> MSKTLMLVKSGLAAGAMGGVALVAGTAQNVAPPPAALAPSYLVKTADSSCADPAWNAAAVYTGGQRVSYQNQTWQAKWWTQGNTPAAGDASPWQLIGQCGGGTPSDPPLVQVPPPTGNALCRPEALAQTQGVDVPYCAVYKQGGAEQLANGSRRRIIGYFTSWRTGKDGSPAYLASDIPWSKLTHINYAFAHVDGSNKLSVNETAPGNPATDMSWPGVAGAEMD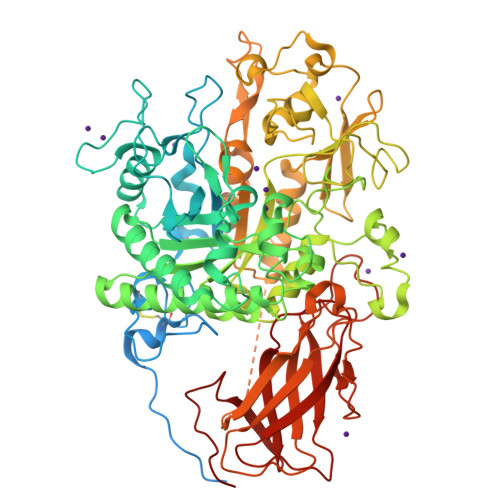ASLPYKGHFNLLTQYKRKYPGVKTLISVGGWAETGGYFDANGKRVASGGFYSMTVNADGTVNQAGINAFSDSAVAFLRKYGFDGVDIDFEYPTSMNNAGNPLDWTFSNARLGSLNKGYVALLQTLRDRLDRAAAQDGRYYQITAAVPASGYLLRGMETFQGLKYLDFVNVMSYDLHGAWNRFVGPNAALYDDGKDAELAFWNVYSTPQYGNIGYLNTDWAYHYYRGGLPASRVNMGVPYYTRGWKNVSGGSNGLWGSSVGSNCPAGLTECGDGAVGIDNIWHDLDDSGKEIPGGSNPMWHAKNLEKGLAGSYLAAYGIDPTLPINQLTGSYQRNYNGALAAPWLWNAGKKVFLSTEDEQSIAQKAAWIDANNVGGVMFWELAGDYDWKAQRNNGQGEYFIGTTLTSLLYNTFSQPPKVSARRADAAPAPTAAIDVGFSLGGFKLGDQNYPINPKLTIVNRSQTTLPGGTEFQFDVPTSAPANIADQSGFGLKVVSAGHSGSNVGGLKGDFNRVSVKLPSWQSLGAGQSVTLDVVYYLPISGPSHYTVGLNGKTYAIRDEAPYLPYLRVL>[2x]HHHHHHSSGLVPRGSHMFRSSLTHLQAASRVFIVGGHITPFVGKGSPLFIDKKHPDFGKKKNMTLEEILATT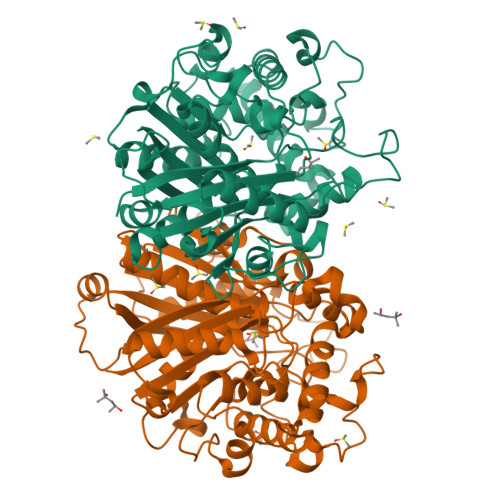VQGTMEHSGLSGREGIVDQVVVGNFLGELFSSQGHLGPAAIGSLTYGQAGSKNPLMYKPAMRVEGASASGGLAVISAMNALKSGSADITLAVGVEVQTTASARVGGDYLARAADYQRQRQLDDFTFPCLFAKRMKYIAEHNHFTMEDTARVAAKAYANGNKNPLAHMHTRKLTFEQCNGEDPSNVKFLGNETYKEYLRMTDCSQVSDGGAGVVLANEEGLRKMGLSPNDSRLVEIKSIACAVSNLYEDPDDACCMFTSRQAAQKALSMANIKPSDLNVAEVHDCFTIAEMLMYEALGIAEYGHAKDLIRNGDTTLEGRIPVNTGGGLLSFGHPVGATGIKQIMEVYRQMKGQCEAYQMKKIPALGATLNMGGDDKTAVSAVLQNI> MDHHHHHHMKVTIPSGKRYYYAGMGITTPGGKVDIADSKKKSKTRIYTESGWFLSDRAIGQGVSGIVPVGTIGQKGDGTISQTLFPEMPTDFKQLSKLETGIHITDDMRGKYLTFAARAINSYGRVGNYQEADRIWIMGLPVTQNVRLHTDADLALLKNGNTTSLIPTDNQLHTNTEVRDYFNDVVYGATIPVLNYKEPAINQTRQLIALDGRTMQFSNHNFNNGYTTSVLIGNRQQTGPLLTYKLDDTLTWGINLENDGRIAIKTVDTTTANNGGQEYIQNVKLDYSNDNSIQVRSAAKNGSLGIEIFINGQSVYNKTVSLTRNRTTHNISSGQIIFGGNTYINEFAVYTESLNNSNIQKLAEYFRDKYKAS

Type 4 pili (T4P)—important in bacterial pathogens—are filaments composed of one well-characterized major pilin, and several minor pilins whose roles are often poorly understood. Streptococcus sanguinis T4P are composed of five pilins, which makes it a good model to determine the role of each pilin subunit in detail. PilE1/PilE2 are the major pilins forming the backbone of the filament, while the three minor pilins (PilA, PilB, and PilC) form a tip-located complex promoting adhesion to various host receptors. Here, we characterize PilA and PilC, showing how they interact and how they function.

To confirm the prediction that PilC might be a modular pilin, we solved its 3D structure by X-ray crystallography. After optimizing the best diffracting crystals and using SeMet protein for phase determination, we solved a high-resolution structure at 1.45 Å. Strikingly, while bioinformatics only predicted that the C terminus of PilC corresponds to a lectin domain, our structure reveals two distinct modules. The first module adopts an Ig-like fold (PilCIg), consisting of two β-sheets packed against each other. The second module that corresponds to the lectin (PilClectin), is a β-sandwich characterized by two opposing antiparallel β-sheets of six strands, with concave and convex sides. PilClectin shows significant structural similarity to multiple carbohydrate-binding proteins, including galectins such as human Gal-7 (PDB 2 GAL). In the Gal-7 structure, the protein interacts with galactose via a carbohydrate-recognition domain (CRD) forming a patch on the concave side of the protein. Since the two proteins share good structural homology in that region, we speculate that the CRD might be on the concave side of PilClectin. When we compared our two PilC structures, we found that they are essentially identical, superposing onto each other with an rmsd of only 0.79 Å. We then purified these mutant proteins and quantified their affinity for 3′-SL using ITC, before comparing it with WT PilC. This revealed that PilCT347A and PilCK349A displayed significantly reduced affinity for 3′-SL, which was particularly pronounced for PilCK349A, with 39.3 ± 1.4% of the WT binding.> GNKWN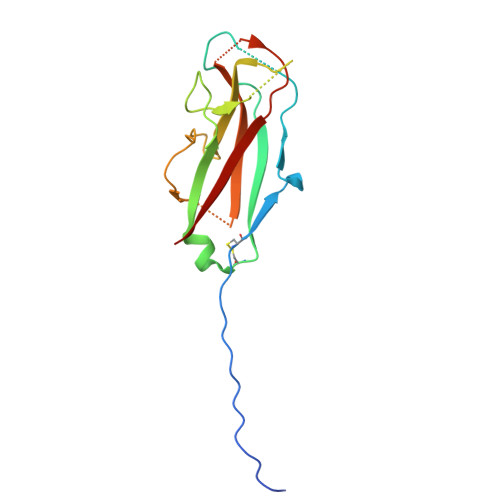TTLPGGNMQFQGVIIAETCRIEAGDKQMTVNMGQISSNRFHAVGEDSAPVPFVIHLRECSTVVSERVGVAFHGVADGKNPDVLSVGEGPGIATNIGVALFDDEGNLVPINRPPANWKRLYSGSTSLHFIAKYRATGRRVTGGIANAQAWFSLTYQ> 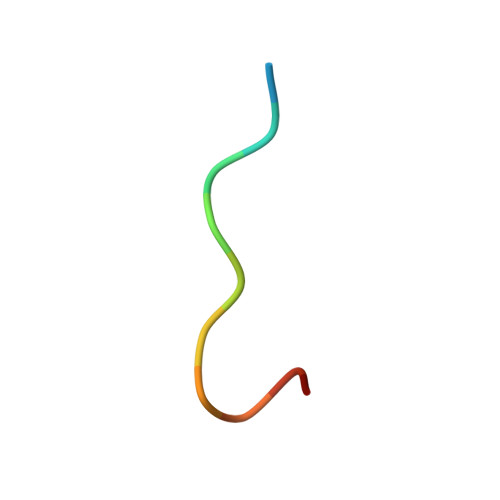XWPPPPTEDELX> EIASEYLGGPGGDAFDDKAVAQNGDITRIEMQCTDVATYIKLRYGKVDSRQWGWGNENCIQWSKKGEKVVHELSSGEYITSAIVTYGKYVQSITFKTNKRTLPRCGTSATEKSVTVL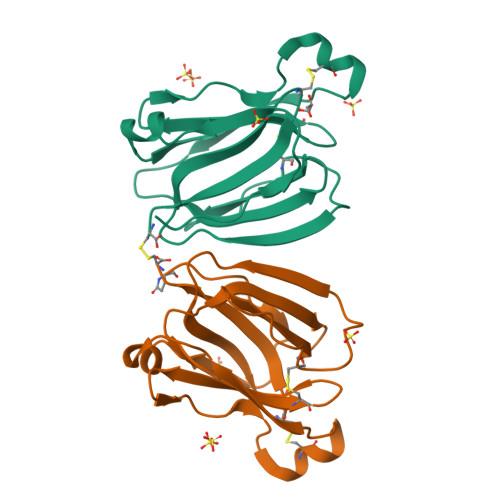IPGGLKYISGRWGCRIDGLRFHAKC;> QVASEYLGGPGGDAFDDKAVAQNGDITRIEMQCTDVATYIKLRYGKVDSRQWGWGNENCIQWSKKGEKVVHELSSGEYITSAIVTYGKYVQSITFKTNKRTLPRCGTSATEKSVTVLIPGGLKYISGRWGCRIDGLRFHAKC> MASW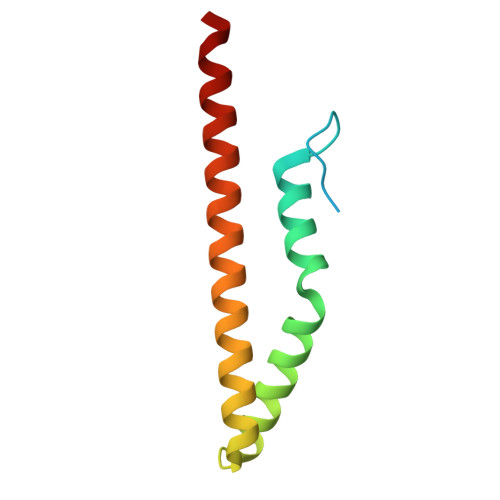SHPQFEKIEGRMSVTVPNDDWTLSSLSETFDDGTQTLQGELTLALDKLAKNPSNPQLLAEYQSKLSEYTLYRNAQSNTVKVIKDVDAAIIQNFR>[4x]GSPEFATMSVSEIFVELQGFLAAEQDIREEIRKVVQSLEQTAREILTLLQGVHQGTGFQDIPKRC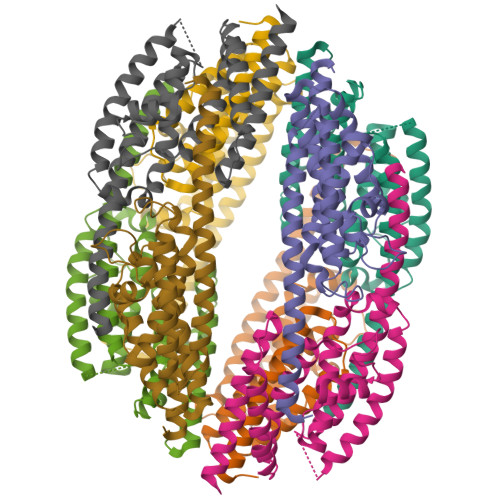LKAREHFSTVKTHLTSLKTKFPAEQYYRFHEHWRFVLQRLVFLAAFVVYLETETLVTREAVTEILGIEPDREKGFHLDVEDYLSGVLILASELSRLSVNSVTAGDYSRPLHISTFINELDSGFRLLNLKNDSLRKRYDGLKYDVKKVEEVVYDLSIRGFNKETAAACGEK> MLDAFSRVVVNSDAKAAYVGGSDLQALKK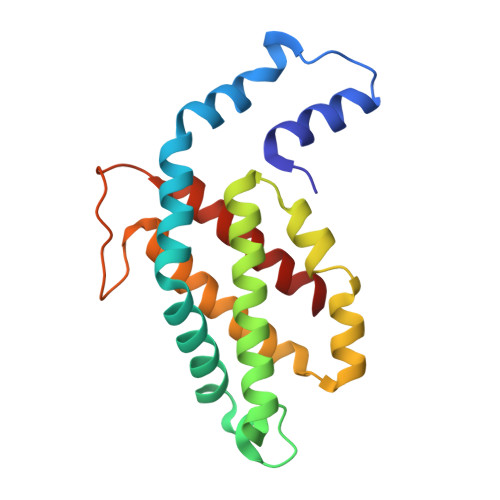FITDGNKRLDSVSFVVSNASCIVSDAVSGMICENPGLIAPGGNCYTNRRMAACLRDGEIILRYASYALLAGDPSVLEDRCLNGLKETYIALGVPTNSSVRAVSIMKASATAFVSGTASDRKMACPDGDCSALASELGSYCDRVAAAIS> GCGUCGCGCC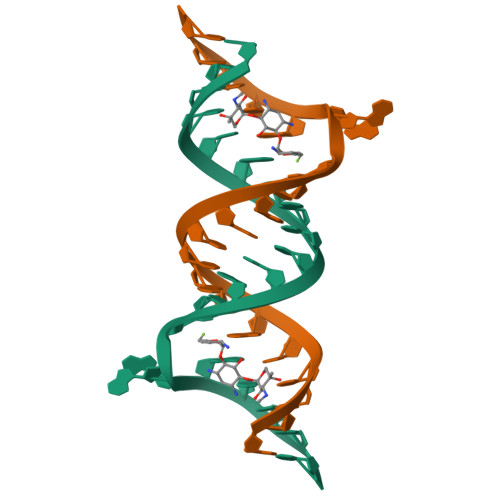GGCGAAGUCGC The basil EGS and petunia IGS are closely related to a number of other NADPH-dependent enzymes that act on phenylpropanoid-derived substrates. Structurally, the PIP-family proteins organize around an N-terminal, Rossman-fold domain, containing a core, six-stranded parallel β-sheet flanked on each face by an α-helical layer. In summary, a mechanistic scheme emerges in which binding of the coniferyl acetate substrate within the active site of EGS leads to deprotonation of the p-hydroxy group (PUSH) coupled with expulsion of acetate ion from the C1 substituent (PULL).

A structure solution was obtained initially for the orthorhombic crystal form of holo-EGS, which contains two EGS/NADP+ complexes per asymmetric unit. A three-dimensional model was refined at 1.7-Å resolution resulting in crystallographic R-factors of 0.244 and 0.267 (working and FreeR, respectively). This refined structure then served as the search model for MR analysis of the monoclinic crystal form. The structures of EGS complexed with NADP+ or NADPH provide the first structural characterization of nicotinamide-cofactor binding by the PIP family of enzymes (previous crystallographic analyses had yielded only apo-enzyme structures). The cofactor is bound through a large number of polar and non-polar interactions. The adenine ring adopts the anti conformation and is sandwiched between the δ-guanido group of Arg39 and the carboxamide group of Gln87. The 2′-phosphate is sequestered by a short loop formed by residues 38–42, and is hydrogen bonded to the side chains of Thr38, Arg39 and Ser42. The nicotinamide ring adopts the anti conformation with its B-face stacked against the side chain of Phe154 and its A-face directed towards the substrate-binding pocket. The nicotinamide carboxamide group forms hydrogen bonds to three backbone atoms (ON7 to 154 N, and NN7 to 112 O and 152 O).

>[2x]SGHGMEENGMKSKILIFGGTGYIGNHMVKGSLKLGHPTYVFTRPNSSKTTLLDEFQSLGAIIVKGELDEHEKLVELMKKVDVVISALAFPQILDQFKILEAIKVAGNIKRFLPSDFGVEEDRINALPPFEALIERKRMIRRAIEEANIPYTYVSANCFASYFINYLLRPYDPKDEITVYGTGEAKFAMNYEQDIGLYTIKVATDPRALNRVVIYRPSTNIITQLELISRWEKKIGKKFKKIHVPEEEIVALTKELPEPENIPIAILHCLFIDGATMSYDFKENDVEASTLYPELKFTTIDELLDIFVHDPPPPASAAF>[2x]GHMVPVVCEVVSEAIVHAAQKLKEYLGFEYPPSKLCPAANTLNEIFLIHFITFCQEKGVDEWLTTTKMTKHQAFLFGADWIWTFWGSDKQIKLQLAVQTLQMSSPPPVESKPCDLSNPESRVEESSWKKSRFDKLEEFCNLIGEDCLGLFIIFGMPGKPKDIRGVVLDSVKSQ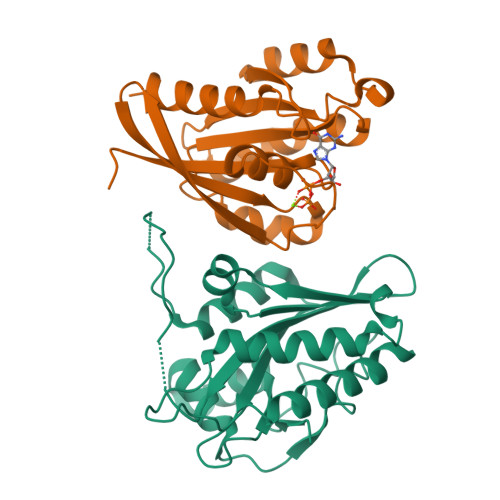MVRSHLPGGKAVAQFVLETEDCVFIKELLRNCLSKKDGLREVGKVYISIL;>MNFDYMFKLLIIGNSSVGKTSFLFRYADDTFTPAFVSTVGIDFKVKTVYRHEKRVKLQIWDTAGLERYRTITTAYYRGAMGFILMYDITNEESFNAVQDWATQIKTYSWDNAQVILVGNKCDMEEERVVPTEKGQLLAEQLGFDFFEASAKENISVRQAFERLVDAICDKMSDS[2x]> ATCDDGRTTANAACCILFPILDDIQENLFDGAQCGEEVHESLRLTFHDAIGFSPTLGGGGADGSIIAFDTIETNFPANAGIDEIVSAQKPFVAKHNISAGDFI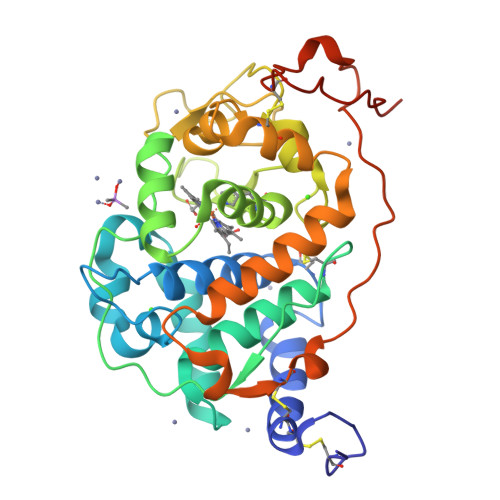QFAGAVGVSNCPGGVRIPFFLGRPDAVAASPDHLVPEPFDSVDSILARMGDAGFSPVEVVWLLASHSIAAADKVDPSIPGTPFDSTPEVFDSQFFIETQLKGRLFPGTADNKGEAQSPLQGEIRLQSDHLLARDPQTACEWQSMVNNQPKIQNRFAATMSKMALLGQDKTKLIDCSDVIPTPPALVGAAHLPAGFSLSDVEQACAATPFPALTADPGPVTSVPPVPGS> MQDNSRYTHFLTQHYDAKPQGRDDRYCESIMRRRGLTSPCKDINTFIHGNKRSIKAICENKNGNPHRENLRISKSSFQVTTCKLHGGSPWPPCQYQATAGFRNVVVACENGLPVHLDQSIFRRP

Angiogenin (ANG), a 14-kDa basic protein is an angiogenic ribonuclease and member of the bovine pancreatic ribonuclease (RNase A) family (also known as RNase 5). Like RNase A, ANG cleaves preferentially on the 3′ side of pyrimidines and follows a transphosphorylation/hydrolysis mechanism. In addition, the crystal structure of human ANG has revealed that it has an RNase A fold and the catalytic triad (residues H13, K40 and H114) is conserved. The enzymatic activity of ANG is several orders of magnitude lower than that of RNase A towards conventional RNase substrates, but essential for its angiogenic effect.

R95 is located on the surface of the molecule in the structure of ANG. It forms part of the β5 strand and interacts with K82 and H84 from the neighboring β4 strand6. Based on previous mutagenesis studies, both K82 and H84 have been shown to have minor roles in catalysis. In the PD variant structure R95Q, the Gln side chain is flexible (can be observed in two possible conformations in the electron density map). However, shortening of the side chain length in the variant seems to have resulted with loss of interactions with H84 thus providing a possible explanation for the diminished catalytic activity of 52%.>MTNATTITMDQGMANQASQAMQIQTYCNSVKQQVPVDFSQFPNLKDNQTQINQGLDLAKGHADLYLNTIQPQIITNISNISNYFALQNAIPAVLPPGSTKAQWLRQLSVIKEQATEYQRLSSDTRLVIVNLNNNLITDSSNFQGIVVNLNSKVQGDNGVLAQLNGDIDKVNAAIDGAIAGIVAGGLLVIGGAFVT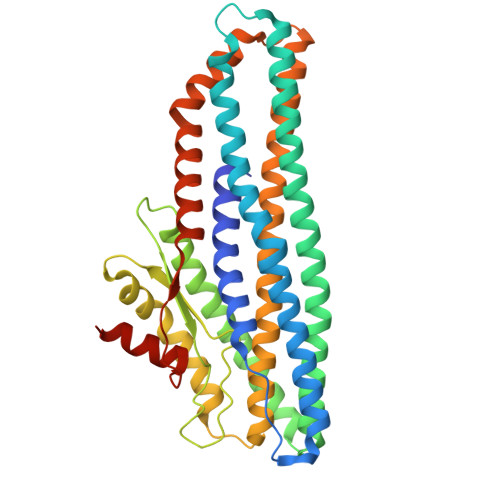AIGAVADFVTAGTSTPVVIGGVAMMVAGAGGITAGAIVLHNSLGARQDLYQKRSSLNSEVLIATQIGNGYKGLQVQAQNAVTAATQMSNAWDSLTSDLGSLITDLDKGITSGDDIRQLWLTAADTTVKTVLTDVTTIKAQMAGVSPLQVPQTDTIANFVARLAALEHHHHHH[3x]>[2x]AHHHHHHGSEIDKGLAKFGDSLINFLYSLALTEFLGKPTGDRVPNASLAIALELTGLSKNLRRVDKHAKGDYAEALIAKAWLMGLI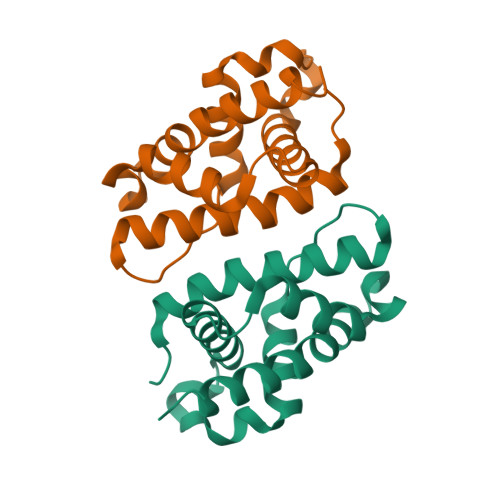SEREAVEIIKKNLYPEVLDFSKKKEAIGRALAPLLVIISERLYSSQV> MGYYDDDAHGHVEADAAPRATTGTGTGSASQTVTIPCHHIRLGDILILQGRPCQVIRISTSAATGQHRYLGVDLFTKQLHEESSFVSNPAPSVVVQTMLGPVFKQYRVLDMQDGSIVAMTETGDVKQNLPVIDQSSLWNRLQKAFESGRGSVRVLVVSDHGREMAVDMKVVHGSRL

Here, we present InCellCryst, an advanced pipeline for producing homogeneous microcrystals directly within living insect cells. We have demonstrated the pipeline on five different proteins (IMPDH, HEX-1, Cathepsin B, Luciferase and EGFP-µNS), representing a selection of soluble proteins of different source organisms that crystallize in insect cells in their native compartment or, in case of peroxisomes, readily in the cytoplasm or nucleus of the cells. Importantly, as shown for IMPDH and HEX-1, InCellCryst can produce crystals from native protein sequences, without purification tags or even remnants of proteolytically removed tags, within a quasi-native cellular environment. The rich source of biomolecules in the cellular environment allows the identification of native ligands by co-crystallization at quasi physiological conditions, representing a unique feature of InCellCryst.

The unmodified HEX-1 crystallizes in blocky hexagons. Even unmodified HEX-1 formed crystals of two different shapes. A predominant hexagonal, block-like morphology that is comparable to, although much larger than, the woronin bodies found in the native fungus, as well as a bipyramidal shape that was not reported to occur natively. Whereas HEX-1 cyto and cyto v2 both formed spindle-like as well as bipyramidal crystals, HEX-1 ori crystals exhibit a hexagonal block shape. For HEX-1 ori and HEX-1 cyto crystals diffracted at 100 K one distinct unit cell population was found, whereas two unit cell populations were identified for HEX-1 cyto v2. For data collection from intact crystal-containing cells at 100 K, we carefully transferred the cells onto a MicroMesh mounted on a light microscope stage. Serial diffraction datasets of the crystals contained in viable cells was performed using a helical grid scan approach, available at the EMBL P14 beamline located at the PETRA III storage ring (DESY, Hamburg, Germany). CrystFEL is optimized for still images in high multiplicity collected at RT at XFEL sources and thus, can be directly applied to serial synchrotron data. All HEX-1 structures show an increased flexibility between Phe145 and Ser151, the C-terminal loop region after the α-helix.6-benzyloxo-2-chloropurine | C12 H9 Cl N4 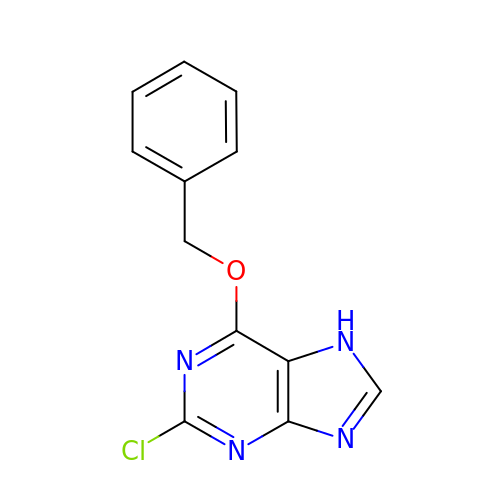O | XKVATRYEPITAPH-UHFFFAOYSA-N>[3x]MANVDEAILKRVKGWAPYVDAKLGFRNHWYPVMFSKEINEGEPKTLKLLGENLLVNRIDGKLYCLKDRCLHRGVQLSVKVECKTKSTITCWYHAWTYRWEDGVLCDILTNPTSAQIGRQKLKTYPVQEAKGCVFIYLGDGDPPPLARDTPPNFLDDDMEILGKNQIIKSNWRLAVENGFDPSHIYIHKDSILVKDNDLALPLGFAPGGDRKQQTRVVDDDVVGRKGVYDLIGEHGVPVFEGTIGGEVVREGAYGEKIVANDISIWLPGVLKVNPFPNPDMMQFEWYVPIDENTHYYFQTLGKPCANDEERKKYEQEFESKWKPMALEGFNNDDIWAREAMVDFYADDKGWVNEILFESDEAIVAWRKLASEHNQGIQTQAHVSGLEHHHHHH;>MNQIWLKVCAASDMQPGTIRRVNRVGAAPLAVY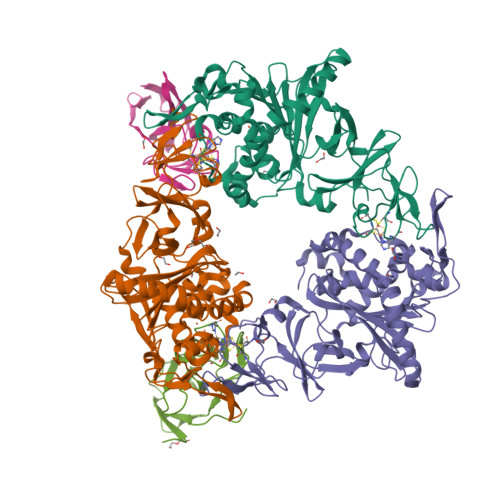RVGDQFYATEDTCTHGIASLSEGTLDGDVIECPFHGGAFNVCTGMPASSPCTVPLGVFEVEVKEGEVYVAGEKKLEHHHHHH[2x]2-AMINOPHENOL | C6 H7 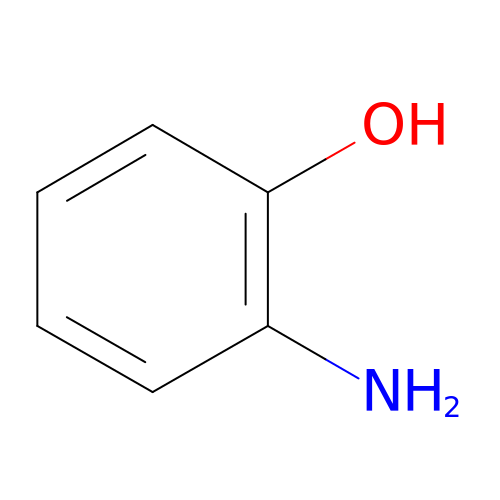N O | CDAWCLOXVUBKRW-UHFFFAOYSA-N>MGDRGSSRRRRTGSRPSSHGGGGPAAAEEEVRDAAAGPDVGAAGDAPAPAPNKDGDAGVGSGHWELRCHRLQDSLFSSDSGFSNYRGILNWCVVMLILSNARLFLENLIKYGILVDPIQVVSLFLKDPYSWPAPCLVIAANVFAVAAFQVEKRLAVGALTEQAGLLLHVANLATILCFPAAVVLLVESITPVGSLLALMAHTILFLKLFSYRDVNSWCRRARAKAASAGKKASSAAAPHTVSYPDNLTYRDLYYFLFAPTLCYELNFPRSPRIRKRFLLRRILEMLFFTQLQVGLIQQWMVPTIQNSMKPFKDMDYSRIIERLLKLAVPNHLIWLIFFYWLFHSCLNAVAELMQFGDREFYRDWWNSESVTYFWQNWNIPVHKWCIRHFYKPMLRRGSSKWMARTGVFLASAFFHEYLVSVPLRMFRLWAFTGMMAQIPLAWFVGRFFQGN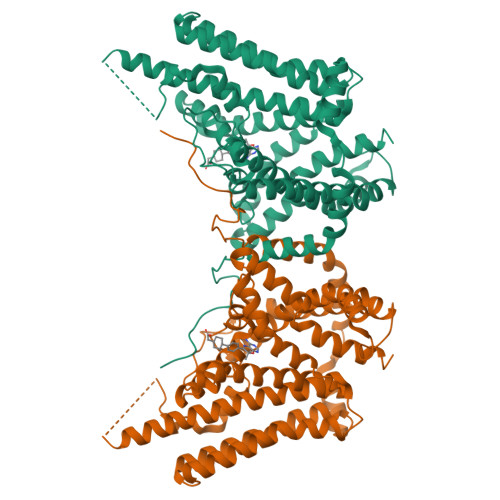YGNAAVWLSLIIGQPIAVLMYVHDYYVLNYEAPAAEA[2x]2-(2,3-DIHYDROXY-BENZOYLAMINO)-3-HYDROXY-PROPIONIC ACID | C10 H11 N 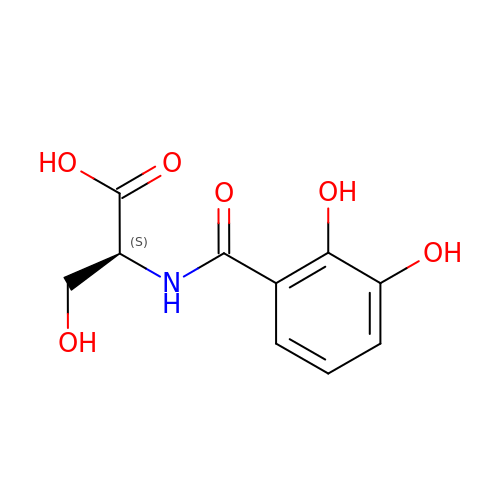O6 | VDTYHTVHFIIEIL-LURJTMIESA-N>XRMKQIEDKIEEIESKQKK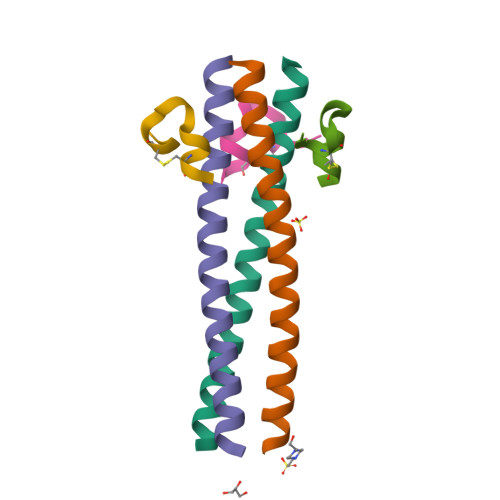IENEIARIKKLLQLTVWGIKQLQARILX[3x];>[3x]XKGACDYPEWQWLCAAX>[3x]MAGAIENARKEIKRISLEDHAESEYGAIYSVSGPVVIAENMIGCAMYELVKVGHDNLVGEVIRIDGDKATIQVYEETAGLTVGDPVLRTGKPLSVELGPGLMETIYDGIQRPLKAIKEESQSIYIPRGIDTPALDRTIKWQFTPGKFQVGDHISGGDIYGSVFENSLISSHKILLPPRSRGTITWIAPAGEYTLDEKILEVEFDGKKSDFTLYHTWPVRVPRPVTEKLSADYPLLTGQRVLDALFPCVQGGTTCIPGAFGCGKTVISQSLSKYSNSDAIIYVGCGERGNEMAEVLMEFPELYTEMSGTKEPIMKRTTLVANTSNMPVAAREASIYTGITLAEYFRDQGKNVSMIADSSSRWAEALREISGRLGEMPADQGFPAYLGAKLASFYERAGKAVALGSPDRTGSVSIVAAVSPAGGDFSDPVTTATLGITQVFWGLDKKLAQRKHFPSINTSVSYSKYTNVLNKFYDSNYPEFPVLRDRMKEILSNAEELEQVVQLVGKSALSDSDKITLDVATLIKEDFLQQNGYSTYDAFCPIWKTFDMMRAFISYHDEAQKAVANGANWSKLADSTGDVKHAVSSSKFFEPSRGEKEVHGEFEKLLSTMQERFAESTD;>MVLSDKELFAINKKAVEQGFNVKPRLNYNTVSGVNGPLVILEKVKFPRYNEIVNLTLPDGTVRQGQVLEIRGDRAIVQVFEGTSGIDVKKTTVEFTGESLRIPVSEDMLGRIFDGSGRPIDNGPKVFAEDYLDINGSPINPYARIYPEEMIS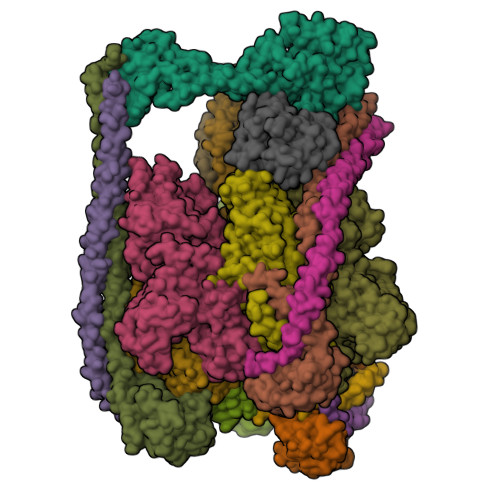TGVSAIDTMNSIARGQKIPIFSASGLPHNEIAAQICRQAGLVRPTKDVHDGHEENFSIVFAAMGVNLETARFFKQDFEENGSLERTSLFLNLANDPTIERIITPRLALTTAEYLAYQTERHVLTILTDMSSYADALREVSAAREEVPGRRGYPGYMYTDLSTIYERAGRVEGRNGSITQIPILTMPNDDITHPIPDLTGYITEGQIFVDRQLHNKGIYPPINVLPSLSRLMKSAIGEGMTRKDHGDVSNQLYAKYAIGKDAAAMKAVVGEEALSIEDKLSLEFLEKFEKTFITQGAYEDRTVFESLDQAWSLLRIYPKEMLNRISPKILDEFYDRARDDADEDEEDPDTRSSGKKKDASQEESLI[3x];>MSSAITALTPNQVNDELNKMQAFIRKEAEEKAKEIQLKADQEYEIEKTNIVRNETNNIDGNFKSKLKKAMLSQQITKSTIANKMRLKVLSAREQSLDGIFEETKEKLSGIANNRDEYKPILQSLIVEALLKLLEPKAIVKALERDVDLIESMKDDIMREYGEKAQRAPLEEIVISNDYLNKDLVSGGVVVSNASDKIEINNTLEERLKLLSEEALPAIRLELYGPSKTRKFFD[3x];>MDYKDDDDKSQKNGIATLLQAEKEAHEIVSKARKYRQDKLKQAKTDAAKEIDSYKIQKDKELKEFEQKNAGGVGELEKKAEAGVQGELAEIKKIAEKKKDDVVKILIETVIKPSAEVHINAL[3x];> MSGNREQVFPTRMTLGLMKTKLKGANQGYSLLKRKSEALTKRFRDITKRIDDAKQKMGRVMQTAAFSLAEVSYATGENIGYQVQESVSTARFKVRARQENVSGVYLSQFESYIDPEINDFRLTGLGRGGQQVQRAKEIYSRAVETLVELASLQTAFIILDEVIKVTNRRVNAIEHVIIPRTENTIAYINSELDELDREEFYRLKKVQEKKQNETAKLDAEMKLKRDRAEQDASEVAADEEPQGETLVADQEDDVIF;> MAEKRTLIAVIADEDTTTGLLLAGIGQITPETQEKNFFVYQEGKTTKEEITDKFNHFTEERDDIAILLINQHIAENIRARVDSFTNAFPAILEIPSKDHPYDPEKDSVLKRVRKLFGE;> MATALYTANDFILISLPQNAQPVTAPGSKTDSWFNETLIGGRAFVSDFKIPEFKIGSLDTLIVESEELSKVDNQIGASIGKIIEILQGLNETSTNAYRTLPINNMPVPEYLENFQWQTRKFKLDKSIKDLITLISNESSQLDADVRATYANYNSAKTNLAAAERKKTGDLSVRSLHDIVKPEDFVLNSEHLTTVLVAVPKSLKSDFEKSYETLSKNVVPASASVIAEDAEYVLFNVHLFKKNVQEFTTAAREKKFIPREFNYSEELIDQLKKEHDSAASLEQSLRVQLVRLAKTAYVDVFINWFHIKALRVYVESVLRYGLPPHFNIKIIAVPPKNLSKCKSELIDAFGFLGGNAFMKDKKGKINKQDTSLHQYASLVDTEYEPFVMYIINL;> MFGVKDAIFKIKRSIAGTDSSDSTAYTTASESSPQLKDSHNPFRNKTTSERTIVEEGSLPPVRLNGYLPSTKNKLLTPEMCDEIRTLMPTRIQLYTEWNLLYSLEQHGSSLHSLYSNVAPDSKEFRRVGYVLVIKDRKNGIFGAYSNEAFHPNEHRQYTGNGECFLWKLDKVPDVNISEKEESEQEGKEGKEEGDKEERWRFSGYPYTGVNEFAIYCTSEFLSMGAGDGHYGLLCDDGLLHGVSNPCQTYGNEVLSKEGKKFSIVALEVWRVG> AQYYPGTTKVAQNRRNFCNPEYELEKLREISDEDVVKILGHRAPGEEYPSVHPPLEEMDEPEDAIREMVEPIDGAKAGDRVRYIQFTDSMYFAPAQPYVRSRAYLCRYRGADAGTLSGRQIIETRERDLEKISKELLETEFFDPARSGVRGKSVHGHSLRLDEDGMMFDMLRRQIYNKDTGRVEMV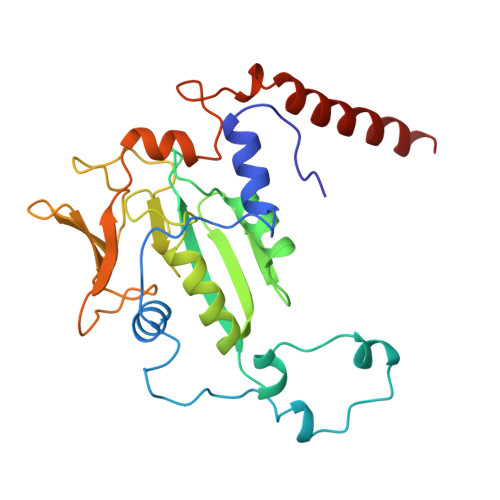KNQIGDELDEPVDLGEPLDEETLMEKTTIYRVDGEAYRDDVEAVEIMQRIHVLRSQGGFNL> HHHHHHHHHHEQKLISEEDLDYKDDDDKMESEMLQSPLLGLGEEDEADLTDWNLPLAFMKKRHCEKIEGSKSLAQSWRMKDRMKTVSVALVLCLNVGVDPPDVVKTTPCARLECWIDPLSMGPQKALETIGANLQKQYENWQPRARYKQSLDPTVDEVKKLCTSLRRNAKEERVLFHYNGHGVPRPTVNGEVWVFNKNYTQYIPLSIYDLQTWMGSPSIFVYDCSNAGLIVKSFKQFALQREQELEVAAINPNHPLAQMPLPPSMKNCIQLAACEATELLPMIPDLPADLFTSCLTTPIKIALRWFCMQKCVSLVPGVTLDLIEKIPGRLNDRRTPLGELNWIFTAITDTIAWNVLPRDLFQKLFRQDLLVASLFRNFLLAERIMRSYNCTPVSSPRLPPTYMHAMWQAWDLAVDICLSQLPTIIEEGTAFRHSPFFAEQLTAFQVWLTMGVENRNPPEQLPIVLQVLLSQVHRLRALDLLGRFLDLGPWAVSLALSVGIFPYVLKLLQSSARELRPLLVFIWAKILAVDSSCQADLVKDNGHKYFLSVLADPYMPAEHRTMTAFILAVIVNSYHTGQEACLQGNLIAICLEQLNDPHPLLRQWVAICLGRIWQNFDSARWCGVRDSAHEKLYSLLSDPIPEVRCAAVFALGTFVGNSAERTDHSTTIDHNVAMMLAQLVSDGSPMVRKEL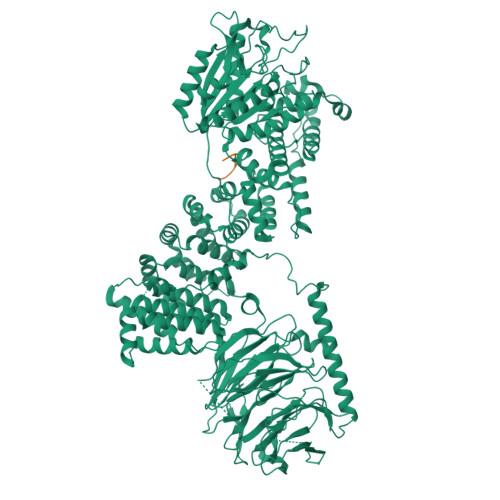VVALSHLVVQYESNFCTVALQFIEEEKNYALPSPATTEGGSLTPVRDSPCTPRLRSVSSYGNIRAVATARSLNKSLQNLSLTEESGGAVAFSPGNLSTSSSASSTLGSPENEEHILSFETIDKMRRASSYSSLNSLIGVSFNSVYTQIWRVLLHLAADPYPEVSDVAMKVLNSIAYKATVNARPQRVLDTSSLTQSAPASPTNKGVHIHQAGGSPPASSTSSSSLTNDVAKQPVSRDLPSGRPGTTGPAGAQYTPHSHQFPRTRKMFDKGPEQTADDADDAAGHKSFISATVQTGFCDWSARYFAQPVMKIPEEHDLESQIRKEREWRFLRNSRVRRQAQQVIQKGITRLDDQIFLNRNPGVPSVVKFHPFTPCIAVADKDSICFWDWEKGEKLDYFHNGNPRYTRVTAMEYLNGQDCSLLLTATDDGAIRVWKNFADLEKNPEMVTAWQGLSDMLPTTRGAGMVVDWEQETGLLMSSGDVRIVRIWDTDREMKVQDIPTGADSCVTSLSCDSHRSLIVAGLGDGSIRVYDRRMALSECRVMTYREHTAWVVKASLQKRPDGHIVSVSVNGDVRIFDPRMPESVNVLQIVKGLTALDIHPQADLIACGSVNQFTAIYNSSGELINNIKYYDGFMGQRVGAISCLAFHPHWPHLAVGSNDYYISVYSVEKRVR;> DEEERVFFMDDVE>[2x]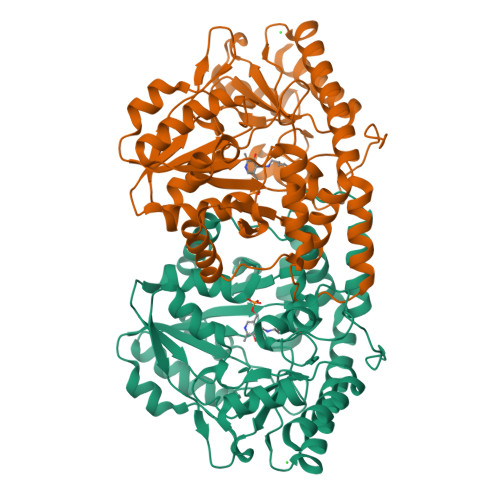SNAMNYNFNEIVDRSNNFSSKWSEMEKKYGTNDLLPMWVADMDFKAAPCIIDSLKNRLEQEIYGYTTRPDSYNESIVNWLYRRHNWKIKSEWLIYSPGVIPAISLLINELTKANDKIMIQEPVYSPFNSVVKNNNRELIISPLQKLENGNYIMDYEDIENKIKDVKLFILCNPHNPVGRVWTKDELKKLGDICLKHNVKIISDEIHSDIILKKHKHIPMASISKEFEKNTITCMAPTKTFNIAGLQSSYVVLPDEKDYKLLDDAFTRIDIKRNNCFSLVATEASYNNGESWLESFLEYLESNIDFAIKYINENMPKLKVRKPEGTYLLWVDFSALGLSDEELESILVQKGKVALNQGNSFGIGGSGYQRINLACPRSMLEEALIRIKNAIN>[6x]MPMISCDMAYGRTDEQKRALSAGLLRVISEATGEPRENIFFVIREGSGINFVEHGEHLPDYVPGNANDKALIAKLK;>[6x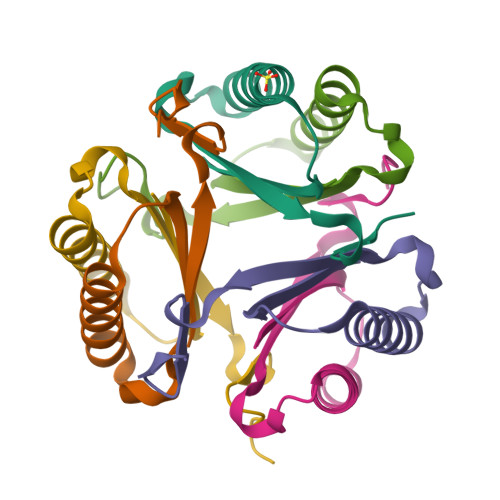]PFIECHIATGLSVARKQQLIRDVIDVTNKSIGSDPKIINVLLVEHAEANMSISGRIHGEAASTERTPAVS> STQYETQGYTINNAGRRLVVDPITRIEGHMRCEVNINDQNVITNAVSCGTMFRGLEIILQGRDPRDAWAFVERICGVCTGVHALASVYAIEDAIGIKVPDNANIIRNIMLATLWCHDHLVHFYQLAGMDWIDVLDALKADPRKTSELAQSLSSWPKSSPGYFFDVQNRLKKFVEGGQLGIFRNGYWGHPQYKLPPEANLMGFAHYLEAL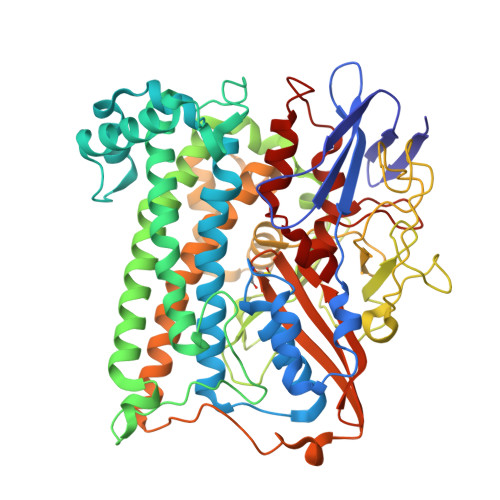DFQREIVKIHAVFGGKNPHPNWIVGGMPCAINIDESGAVGAVNMERLNLVQSIITRTADFINNVMIPDALAIGQFNKPWSEIGTGLSDKCVLSYGAFPDIANDFGEKSLLMPGGAVINGDFNNVLPVDLVDPQQVQEFVDHAWYRYPNDQVGRHPFDGITDPWYNPGDVKGSDTNIQQLNEQERYSWIKAPRWRGNAMEVGPLARTLIAYHKGDAATVESVDRMMSALNLPLSGIQSTLGRILCRAHEAQWAAGKLQYFFDKLMTNLKNGNLATASTEKWEPATWPTECRGVGFTEAPKGALGHWAAIRDGKIDLYQCVVPTTWNASPRDPKGQIGAYEAALMNTKMAIPEQPLEILRTLHSFDPCLACSTH>MRQVDAATHGGRAVIELREKILSGELPGGMRLFEVSTAELLDISRTPVREALSRLTEEGLLNRLPGGGFVVRRFGFADVVDAIEVRGVMEGTAARLAAERGVSKVALEEIDATVQQLDLCFGDRVDDVDFDGYAALNRIFHHQLAALCGSEMIRREVERASSLPFASPSAFLPDKANIGAFRRSLRGAQEQHKAIVAAIVAREGARAEAVAREHSRTARTNLEYMIREAPELIAQVPGLALISDHHHHHH[4x]

Here, we characterized Atu1419 as a transcriptional repressor of its own repression in addition to two other genes (atu1418 and atu1420). The structures revealed Atu1419 to be a member of the VanR group of the FadR C-terminal domain (FCD; Pfam PF07729) subfamily of the large GntR superfamily of transcriptional factors (>93 135 members in Pfam database). Like FadR, Atu1419 possesses a characteristic molecular architecture, composed of a conserved N-terminal DNA binding domain containing the wHTH motif and a C-terminal effector binding/oligomerization domain. We identified the short palindromic region composed of 10 base pairs and a degenerated palindrome bound to Atu1419 and the N5,N10-methylenetetrahydrofolate (MEF) as the effector molecule disrupting Atu1419-DNA interaction, allowing the expression of the second part of the HCA degradation pathway.

We solved the first structure of Atu1419 from crystals grown in sodium citrate buffer using SAD method at the peak absorption energy of Zinc at 2 Å resolution in the space group P212121. Four molecules (A, B, C and D) are present in the asymmetric unit and form a tetramer (a dimer of dimer), which is consistent with the observation that Atu1419 is a tetramer in solution. Remarkably, the four subunits within the tetramer are not identical: molecule A shows large conformational changes as indicated by an average root mean square deviation (RMSD) of 1.28 Å for all Cα atoms compared with the subunits B/C/D, which are more similar (average RMSD of 0.7 Å for all Cα atoms). This is due to the presence of a citrate originated from the crystallization condition, which binds molecule A in the effector binding site in a different orientation (orientation A) than that for citrates in subunits B/C/D (orientation B), which bind similarly. In molecule A, the Cα atoms of Ser169, Lys175 and Arg183 are respectively, 0.92, 6.84 and 7.34 Å away from those in molecules B/C/D, allowing the side chains of Lys175, Arg183 and the NH main chain of Ser169 to interact with the citrate molecule. These latter protein-citrate interactions cannot exist in subunits B/C/D. Nonetheless, all bound citrates share interactions with Arg86, Tyr133, Asn137, His141, His214, Asn221 and a Zn2+ ion that co-purified with Atu1419. Thirteen polar interactions are observed between monomer A and the citrate molecule (orientation A), which is buried within the monomer, leaving only 26.6 Å2 or 8.4% of the molecule surface exposed to solvent. In contrast, there are only ten polar interactions between monomers B/C/D and the citrate with a similar buried surface area. In the case of Atu1419, the citrate in orientation A bound in the effector binding pocket induces large conformational changes from the C-terminal domain to the N-terminal domain. It affects four different protein regions: the wing of the DNA binding domain and three regions of the effector binding domain including the C-terminus protein which is in contact with the DNA binding domain.>[2x]MAHHHHHHMMSLAIEAVKDFLVKLQDDICEALEAEDGQATFMEDKW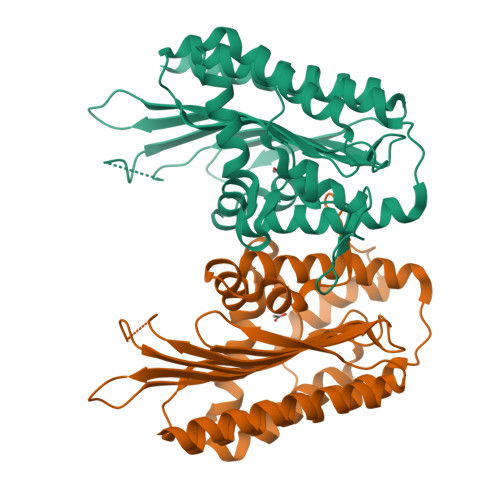TREGGGGGRTRVMVNGAVIEKGGVNFSHVYGKGLPGSSTERHPDMTGCNFQAMGVSLVIHPKNPHVPTSHANVRLFVAEREGKEPVWWFGGGFDLTPYYAVEEDCRYFHQVAQDLCKPFGADVYTRFKVWCDEYFFIPYRNEARGIGGLFFDDLNEWPFEKCFEFVQAVGKGYIDAYIPIVNRRKNTPYTEQQVEFQEFRRGRYAEFNLVIDRGTKFGLQSGGRTESILISLPPRARWGYDWQPEPGTPEARLTEYFLMKRQWV> MVQAV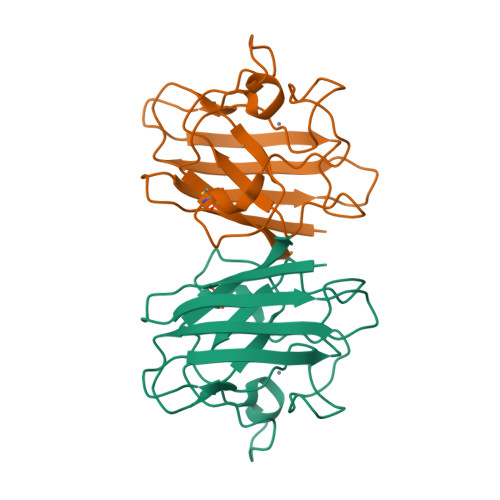AVLKGDAGVSGVVKFEQASESEPTTVSYEIAGNSPNAERGFHIHEFGDATNGCVSAGPHFNPFKKTHGAPTDEVRHVGDMRNVKTDENGVAKGSFKDSLIKLIGPTSVVGRSVVIHAGQDDLGKGDTEESLKTGNAGPRPACGVIGLTN The most abundant virulence factor secreted by Hc yeast cells is Calcium Binding Protein 1 (Cbp1), which is absolutely required for macrophage lysis. The mature secreted form of Cbp1 is 78 amino acids in length, has no known domains, and, prior to this work, had only one known homolog in the closely related fungus Paracoccidioides. The Cbp1 structures displayed an alpha-helical dimer arrangement with an intermolecular four-helix bundle fold at the core formed from the 3rd and 4th helices of each monomer, creating a binocular shape, and thus we dubbed this new arrangement as a “binocular” fold. For both Pb03 and H88 Cbp1, the three disulfide bonds present in each monomer orient the alpha helices so that the aromatic residues (Phe12, Phe19, Trp30) are packed in the interior of the protein, creating the hydrophobic core.

Crystals of Hc H88 and Pb03 Cbp1 homologs formed after a week and diffracted to 1.6 Å. The diffraction data from Hc H88 was resolved by molecular replacement using the Pb03 model. Using this model in the Phaser program in the Phenix crystallography programming suite, we obtained a TFZ score of 8.4 and an LLG score of 63.271, supporting the validity of the molecular replacement solution. The asymmetric unit for the Pb03 Cbp1 crystal contained a single dimer, whereas the asymmetric unit for the H88 crystal contained a dimer of dimers. An alignment of the two dimers of H88 Cbp1 structure gave a root mean squared deviation (RMSD) value of 0.755 Å, indicating the structure remains largely unchanged amongst the dimers. An alignment of the Pb03 and the Hc CBP1 dimers gave an RMSD of 1.6 Å, indicating the structures of the distinct homologs are conserved. The H88 structure was not as clearly polarized but did display a groove of strong negative charge on its C-terminal side. The bottom of the C-terminal helices that form the core four-helix bundle of the Pb03 Cbp1 are much more negative relative to the Hc H88 Cbp1 homolog. When the new structures were aligned against the G186AR NMR structure, the resulting RMSD value was 5.6 Å and 5.8 Å for Pb03 and H88 Cbp1, respectively, consistent with the NMR structure not being found by DALI and VAST searches of the crystal structures. Notably, when we modeled these residues on the Pb03 or H88 crystal structure, we found that the residues that were required for Cbp1 protein secretion were all facing inwards away from the protein surface, suggesting they are important for proper folding.

>DQPSVGDAFDKYNEAVKVFTQLSSAANCDWPACLSSLSASSAACIAAIGELGLDIPLDLACAATATTSATQACKGCLW[4x]>[2x]MRSRRVDVMDVMNRLILAMDLMNRDDALRVTGEVREYIDTVKIGYPLVLSEGMDIIAEFRKRFGCRIIADF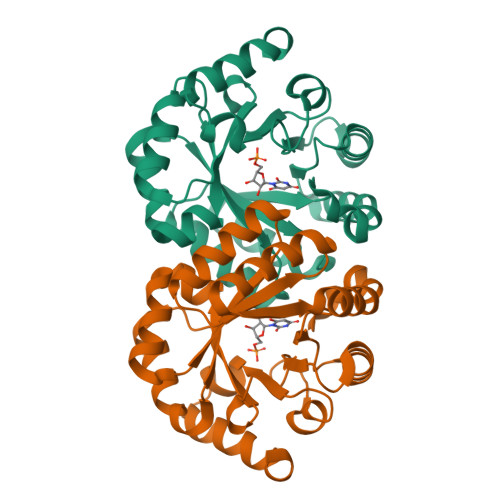KVADIPETNEKICRATFKAGADAISVHGFPGADSVRACLNVAEEMGREVFLLTEMSHPGAEMFIQGAADEIARMGVDLGVKNYVGPSTRPERLSRLREIIGQDSFLISPGVGAQGGDPGETLRFADAIIVGRSIYLADNPAAAAAGIIESIKDLLNP>MSATLLSPLSTHVLNAAQGVPGANMTIVLHRLDPVSSAWNILTTGITNDDGRCPGLITKENFIAGVYKMRFETGKYWDALGETCFYPYVEIVFTITNTSQHYHVP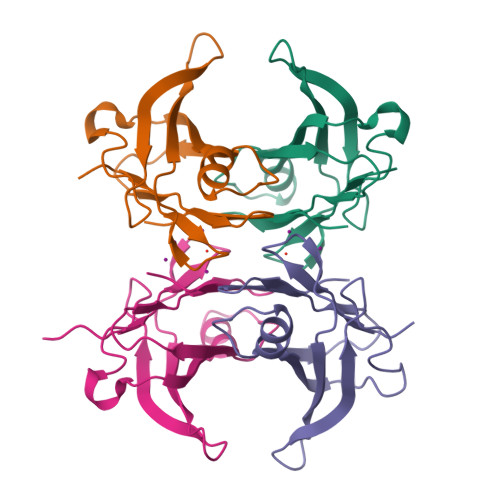LLLSRFSYSTTRGS[4x]> IRCFITPDITSKDCPNGHVCYTKTWCDAFCSIRGKRVDLGCAATCPTVKTGVDIQCCSTDN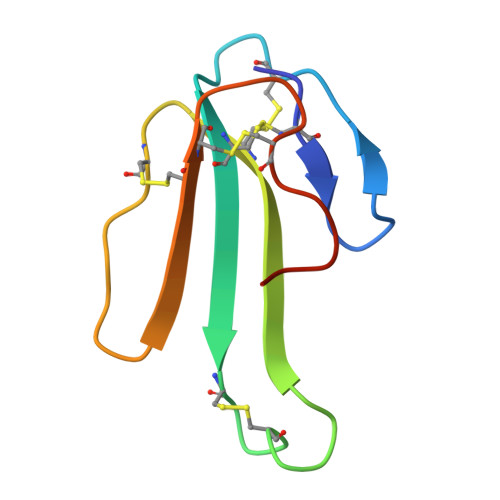CNPFPTRKRP> TRY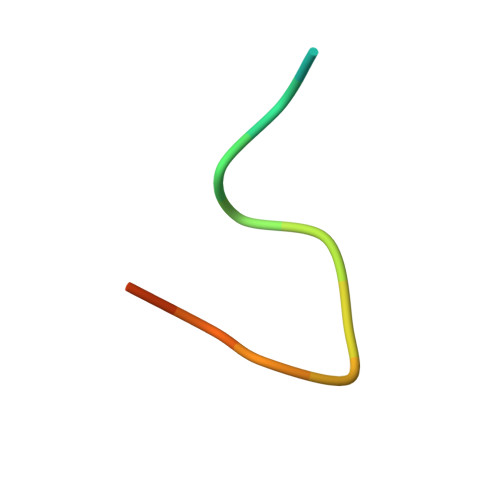ANPKMKPFIFGAX> MALLTPIPSPMVNLTQVIDPTEQLAYFPKITFERLKNYDTSSNYAKGKLTRNYMILLPWQHVNRYNFVFSSTGCKVSLKTCIGKLMKDLNPKVLYFIGEGAGNWMARTACEYPDIKFVYRSLKDDLDHHYPLEYQRVIGELSRIIDSGEGLSMETTDATQKTHWDLIHRVSKDALLITLCDAEFKDRDDFFKMVILWRKHVLSCRICTTYGTDLYL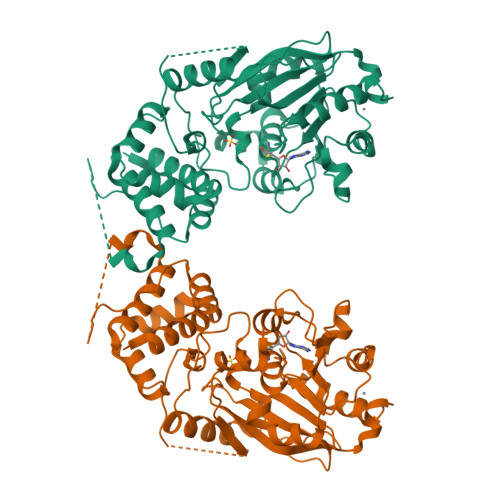FAKYHAKDCNVKLPFFVRSVATFIMQGSKLSGSECYILLTLGHHNNLPCHGEIQNSKMKIAVANDFYAAKKLDNKSIEANCKSLLSGLRIPINKKELNRQRRLLTLQSNHSSVATVGGSKVIESKWLTNKANTIIDWLEHILNSPKGELNYDFFEALENTYPNMIKLIDNLGNAEIKKLIKVTGYMLVSKKSGHHHHHH> SGDGKTS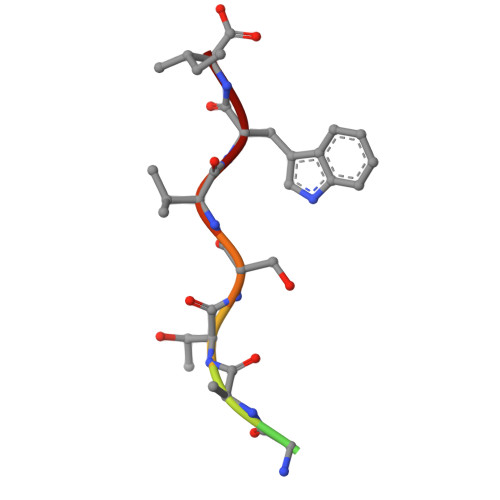VWI>GPGSGDQLGEAKASGNLGNTLKVLGNFDEAIVCCQRHLDISRELNDKVGEARALYNLGNVYHAKGKSFGCPGPQDTGEFPEDVRNALQAAVDLYEENLSLVTALGDRAAQGRAFGNLGNTHYLLGNFRDAVIAHEQRLLIAKEFGDKAAERRAYSNLGNAYIFLGEFETASEYYKKTLLLARQLKDRAVEAQSCYSLGNTYTLLQDYEKAIDYHLKHLAIAQELKDRIGEGRACWSLGNAYTALGNHDQAMHFAEKHLEISREVGDLEVLFQGPPDEDFFDILVKCQGSRLDDQRCAPPSA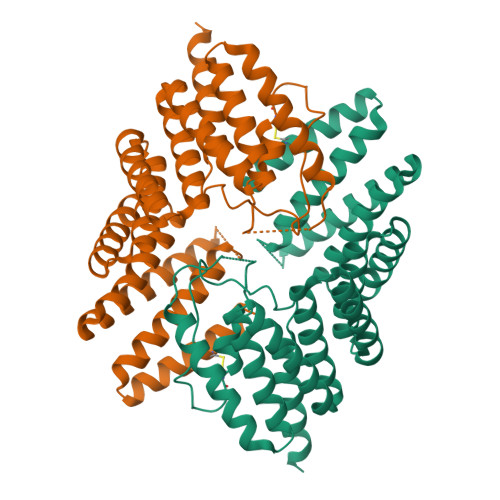ATKGPTVPDEDFFSLILRSQAKRMDEQRVLLQ[2x]>SMQRTVAHQITLLECVGKGRYGEVWRGSWQGENVAVKIFSSRDEKSWFRETELYNTVMLRHENILGFIASDMTSRHSSTQLWLITHYHEMGSLYDYLQLTTLDTVSCLRIVLSIASGLAHLHIEIFGTQGKPAIAHRDLKSKNILVKKNGQCCIADLGLAVMHSQSTNQLDVGNNPRVGTKRYMAPEVLDETIQVDCFDSYKRVDIWAFGLVLWEVARRMVSNGIVEDYKPPFYDVVPNDPSFEDMRKVVCVDQQRPNIPNRWFSDPTLTSLAKLMKECWYQNPSARL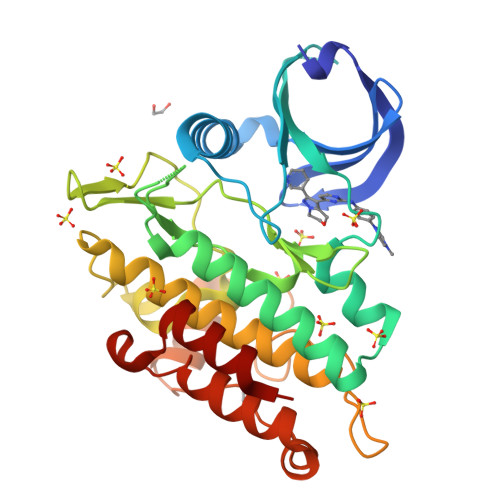TALRIKKTLTKID[2x]>M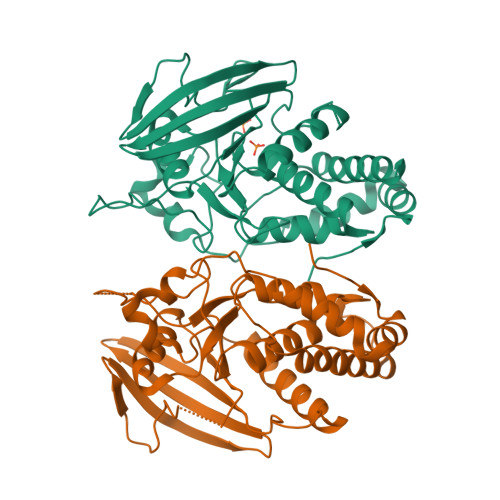SLTNPVQLDDFDAYIKDMAKDSDYKFSLQFEELKLIGLDIPHFAADLPLNRCKNRYTNILPYDFSRVRLVSMNEEEGADYINANYIPGYNSPQEYIATQGPLPETRNDFWKMVLQQKSQIIVMLTQCNEKRRVKCDHYWPFTEEPIAYGDITVEMISEEEQDDWACRHFRINYADEMQDVMHFNYTAWPDHGVPTANAAESILQFVHMVRQQATKSKGPMIIHCSAGVGRTGTFIALDRLLQHIRDHEFVDILGLVSEMRSYRMSMVQTEEQYIFIHQCVQLMWMKKKEGHHHHHH[2x]Here, a highly sample-efficient methodology to measure serial crystallography data from microcrystals by raster scanning within standard in situ 96-well crystallization plates is described. Structures were determined from very small quantities of microcrystal suspension and the results were compared with those from other sample-delivery methods. We demonstrate that raster-scan serial data collection within crystallization plates can be an easily accessible and rapid method of assessing microcrystallization experiments and determining suitable-quality room-temperature structures.

DtpAa crystallized in the monoclinic space group P21, representing a much lower symmetry than was the case for HEWL (P43212) and making it an important test system for the general applicability of this method. Data from an additional 27 drops were added to provide a much higher quality data set (increasing the number of merged diffraction patterns to 22 854), although a total of 35 drops is not very efficient for screening if every tested crystallization condition requires 35 drops for low-symmetry space groups. More amino acids, water molecules and alternate conformations could be convincingly modelled when 35 drops were merged (22 854 merged diffraction patterns), although these were removed for the 12-drop and eight-drop data sets (10 054 and 5360 merged diffraction patterns, respectively) where the electron density was not as clear. The resolution achieved in the fixed-target experiment was 1.78 Å (8596 merged diffraction patterns; Ebrahim et al., 2019), while the in-plate data from 35 drops reached 1.79 Å resolution (22 854 merged diffraction patterns). In previous structures free of radiation-induced changes (measured with 10 fs XFEL pulses) the Fe—OH2 bond length has consistently been shown to be ∼2.4 Å and to progressively increase in a quasi-linear manner with accumulated dose until the water molecule is at a distance that indicates complete dissociation from the heme subsequent to reduction of iron from the ferric to the ferrous state. The observed Fe—O distances of 2.6–2.7 Å in the structures presented here are similar to those observed at doses of 75–100 kGy in experiments where a sequence of still diffraction patterns were obtained from each microcrystal in a fixed target over several tens of milliseconds, providing a fine-grained dose series. The dose delivered in this data collection from crystallization plates was approximately 18 kGy per crystal (and hence for the full data set as each crystal is assumed to be exposed only once), which is significantly lower than would be expected for the observed Fe—O bond length when compared with the SSX data. The doses calculated for in-plate data collection appeared to be lower than suggested by the electron density, although it is important to note that time regimes and sample environments differ from those in the previous fixed-target experiment.

>[2x]DPAGADAGSAVPFHGAHQAGIATPVQDRLHFAAFDVTTEDRAAFVALLKEWTAAARRLTAGHAVGEGAYGGLPEAPPDDTGEALGLKPSRLTLTIGFGPSLFTRFGLADLRPEALADLPKFPGDNLDRARSGGDLCVQACADDPQVAVHAIRNLARIGFGKVVVRWSQLGFGKTSSTTPDKQTPRNLLGFKDGTRNIAGTEKDRLDRFVWAAEKDGTPWMTGGSYLVARRIRMHIETWDRASLQEQEDVFGRDKGEGAPVGKAKERDEPFLKAMKPDAHVRLAHPDSNGGATLLRRGYSFTDGTDGLGRLDAGLFFLAYQRDIRTGFVPVQRNLATDALNEFIQHVGSAVFAVPPGVRDADDWWGSTLFGKEA(9Z)-11-[(2R,3S)-3-pentyloxiran-2-yl]undec-9-enoic acid | C18 H32 O3 | 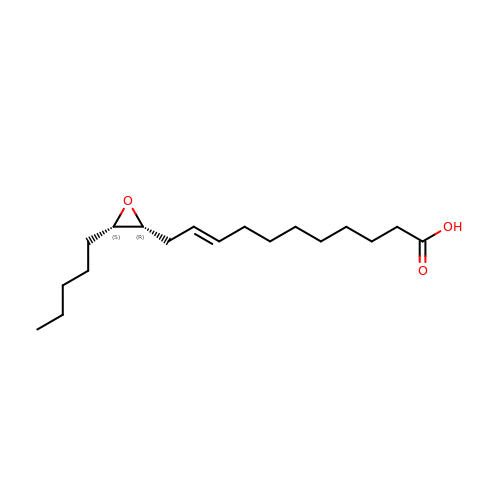CCPPLLJZDQAOHD-BEBBCNLGSA-N>MVPAPEAIRQALQERLLARLDHPDPLYRDLLQDYPRRGGKMLRGLLTVYSALAHGAPLEAGLEAATALELFQNWVLVHDDIEDGSEERRGRPALHRLHPMPLALNAGDAMHAEMWGLLAEGLARGLFPPEVLLEFHEVVRRTAYGQHLDLLWTLGGTFDLRPEDYFRMVAHKAAYYTAVAPLRLGALLAGKTPPAAYEEG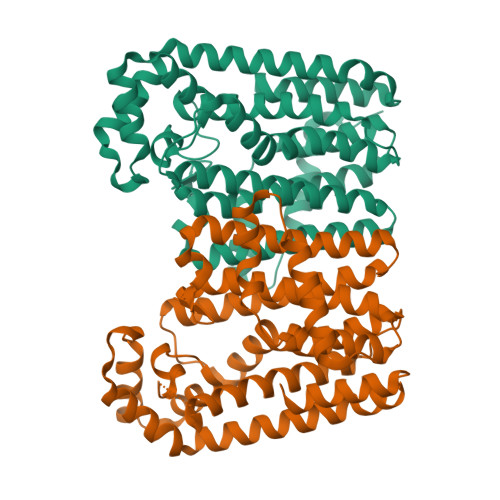GLRLGTAFQIVDDVLNLEGGEAYGKERAGDLYEGKRTLILLRFLEEAPPEERARALALLALPREAKPEAEVGWLLERLLASRALAWAKAEAKRLQAEGLALLEAAFQDLPGKEALDHLRGLLAALVERRA[4x]> FNLISEKCDILSILRDHPENRIYRRKIEELSKRFTAIRKTKGDRNCFYRALGYSYLESLLGKSREIFKFKERVLQTPNDLLAAGFEEHKFRNFFNAFYSVVELVEKDGSVSSLLKVFNDQSASDHIVQFLRLLTSAFIRNRADFFRHFIDEEMDIKDFCTHE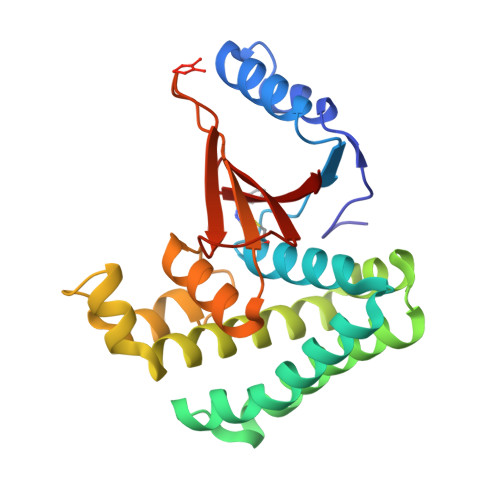VEPMATECDHIQITALSQALSIALQVEYVDEMDTALNHHVFPEAATPSVYLLYKTSHYNILYA2-[2-(2-octoxyethoxy)ethoxy]ethanol 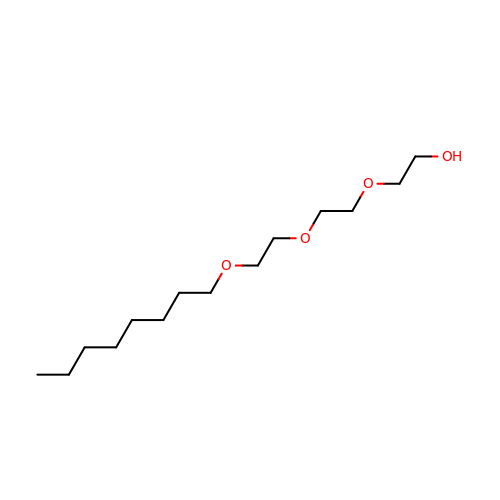| C14 H30 O4 | XIVLVYLYOMHUGB-UHFFFAOYSA-N> GAMIESSTTIQVISAGLPRTGTKSLKNALEIIYHKPCYHMFEIIFNKQSDIIKWQNLIHDSHMITTPPPLTTKTIAIYDKLKELLDGYIATTDLPT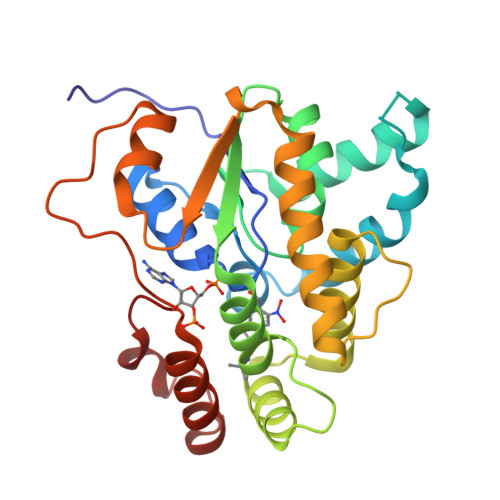CGFYKDLMNIYPNAKVLLTIRDKYDWLHSLRKVVLPKSNDPWKLKIEEGDKVLGLNSDFYKLTEDSLKFAFQKDDLNFDDDQVLLECYDEYNRLVQETVPSDRLLVLRLGDGWEPLCKFLNVEIPNGIDYPCVNSHHQMTQLTEQLIKYKSLDAIIHMFPDLI3,6-Bis{3-[(2R)-2-methylpiperidino)]propionamido}acridine | C31 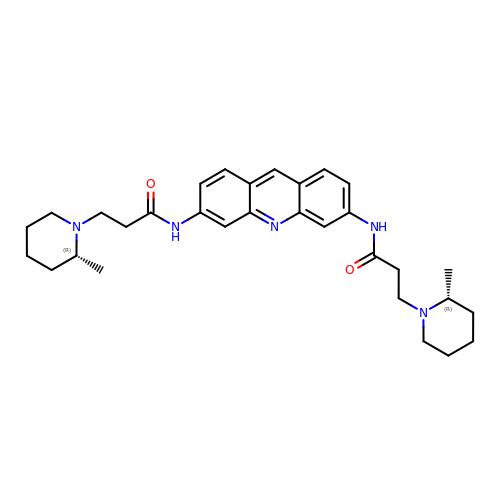H41 N5 O2 | AFTOIBDEHJTNKF-DHIUTWEWSA-N>MAAPSPTTTAAAAAAATTHHRVLLPSARPRAAPSSLRLPLRAQPHAHAHAQRARLAAPVAAAAPAPAASTASPESPASGAVAGKPTVLVAEKLGAAGLALLREFANVDCSYGLSPEDLRAKISLCDALIVRSGTKVGRDVFEASGGRLRVVGRAGVGIDNVDLAAATEHGCLVVNAPTANTVAAAEHGIALLTAMARNIAQADASLKAGKWQRNKYVGVSLVGKTLAILGFGKVGSEVARRAKGLGMHVIAHDPYASADRARAIGVELVSMEEAMTTADFISLHMPLTPATDKMLNDEAFAKMKKGVRIINVARGGVIDEEALVRALDSGVVAQAALDVFTKEPPAADNKLVLHGNVTVTPHLGASTVEAQEGVAIEIAEAVIGALK[2x]

Here, we cloned and functionally characterized the maize (Zea mays) gene Dek20, which encodes phosphoglycerate dehydrogenase1 (PGDH1), the rate-limiting enzyme in the phosphorylated pathway of serine biosynthesis (PPSB). The first step, catalyzed by 3-phosphoglycerate dehydrogenase (PGDH), oxidizes 3-PGA into 3-phosphohydroxypyruvate (3-PHP) and is the rate-limiting reaction. The mature transcript of Dek20 features an 1,881-bp coding sequence, which encodes a protein consisting of 626 amino acids that includes 3 domains: the substrate binding domain (SBD, residues 1-179), the nucleotide-binding domain (NBD, residues 180-367), and the regulatory domain (RBD, residues 388-626). DEK20 and its mammalian homologs are classified as type I PGDH, characterized by 3 major domains: the substrate binding domain, nucleotide-binding domain, and regulatory domains.

To elucidate the molecular mechanism underlying enzymic activity, we first purified the full-length DEK20 for crystallization. However, no crystal was obtained due to relatively flexible interactions between RBD and SBD. Consequently, we purified a truncated version (residues 1-387, referred to as DEK20WT), which includes only the SBD and the NBD. DEK20WT forms a homodimer, with each monomer composed of 1 NBD and 1 SBD. Both domains exhibit conserved architectures: the SBD contains 5 α helices and 5 β strands, while the NBD consists of 7 α helices surrounding a central β sheet. Indeed, both the superimposed cofactor (NAD+/NADH) and the substrate (3-PGA) from human 3-phosphoglycerate dehydrogenase fit well within our structure. The 3-PGA is situated in a cleft between NBD and SBD, stabilized by a series of positive residues such as arginine and histidine, while NAD+ occupies the binding pocket formed by the NBD. Interestingly, a conserved residue His at 284 among different species was located between NAD+ and Ser282. In the structure of DEK20WT, Ser282 formed a hydrogen bond with His284 (3.2 Å) keeping the imidazole group of histidine away from NAD + . Correspondingly, the decreased enzyme activity of DEK20(S282L) was also restored by the H284A mutation. These findings demonstrate that Ser282 is critical for enzyme activity, facilitating its interaction with His284 to keep His284 away from the cofactor, NAD+.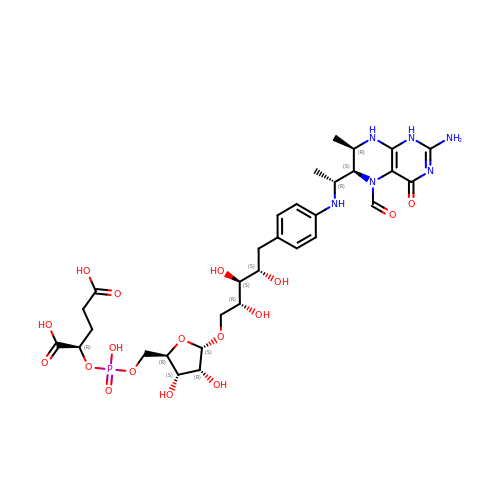1-[4-({(1R)-1-[(6S,7R)-2-amino-5-formyl-7-methyl-4-oxo-1,4,5,6,7,8-hexahydropteridin-6-yl]ethyl}amino)phenyl]-1-deoxy-5-O-{5-O-[(R)-{[(1R)-1,3-dicarboxypropyl]oxy}(hydroxy)phosphoryl]-alpha-D-ribofuranosyl}-D-ribitol | C31 H45 N6 O17 P | RMPHWTMYCVTPKB-DSWDSYRTSA-N>[2x]SMQEKIMRELHVKPSIDPKQEIEDRVNFLKQYVKKTGAKGFVLGISGGQDSTLAGRLAQLAVESIREEGGDAQFIAVRLPHGTQQDEDDAQLALKFIKPDKSWKFDIKSTVSAFSDQYQQETGDQLTDFNKGNVKARTRMIAQYAIGGQEGLLVLGTDHAAEAVTGF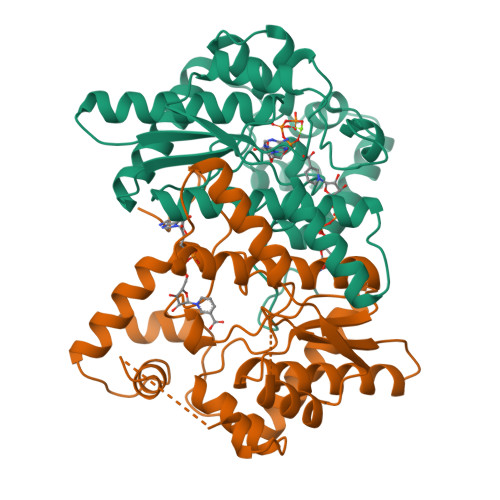FTKYGDGGADLLPLTGLTKRQGRTLLKELGAPERLYLKEPTADLLDEKPQQSDETELGISYDEIDDYLEGKEVSAKVSEALEKRYSMTEHKRQVPASMFDDWWK>EERNDWHFNIGAMYEIENVEGYGEDMDGLAEPSVYFNAANGPWRIALAYYQEGPVDYSAGKRGTWFDRPELEVHYQFLENDDFSFGLTGGFRNYGYHYVDEPGKDTANMQRWKIAPDWDVKLTDDLRFNGWLSMYKFANDLNTTGYADTRVETETGLQYTFNETVALRVNYYLERGFNMDDSRNNGEFSTQEIRAYLPLTLGNHS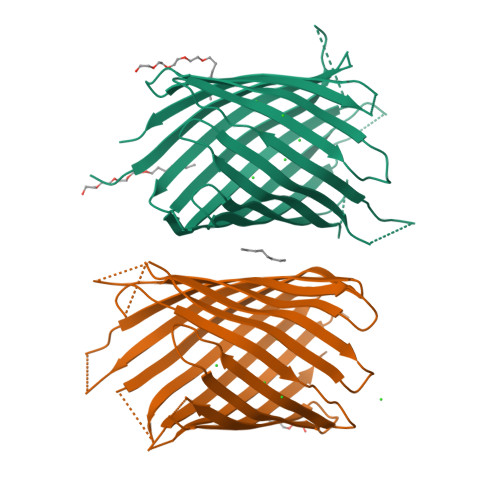VTPYTRIGLDRAGHDFNRVGLFYGYDFQNGLSVSLEYAFEWQDHDEGDSDKFHYAGVGVNYSFHHHHHH[2x]> GFF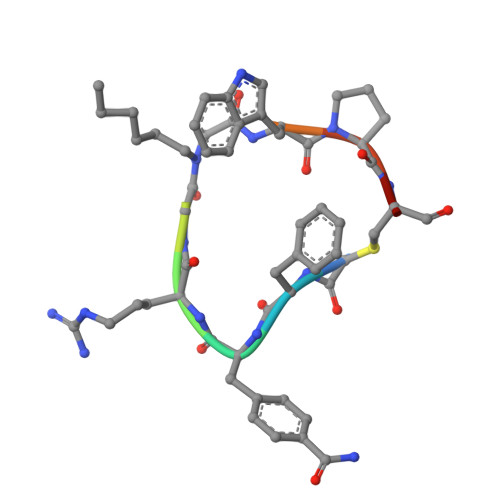RGXWPCG> ALPQTVRIGTDTTAAPFSSKDAKGEFIGFDIDLGNEMCKRMQVKCTWVASDFDALIPSLKAKKID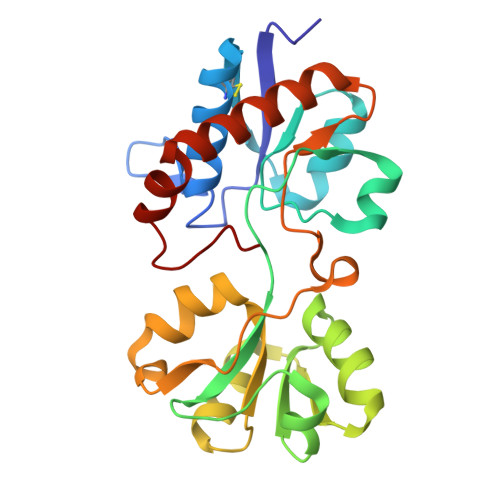AIISSLSITDKRQQEIAFSDKLYAADSRLIAAKGSPIQPTLESLKGKHVGVLQGSTQEAYANDNWRTKGVDVVAYANQDLIYSDLTAGRLDAALQDEVAASEGFLKQPAGKEYAFAGPSVKDKKYFGDGTGVGLRKDDTELKAAFDKALTELRQDGTYDKMAKKYFDFNVYGD> AMAQIDLNITCRFAGVFHVEKNGRYSISRTEAADLCKAFNSTLPTMAQMEKALSIGFETCRYGFIEGHVV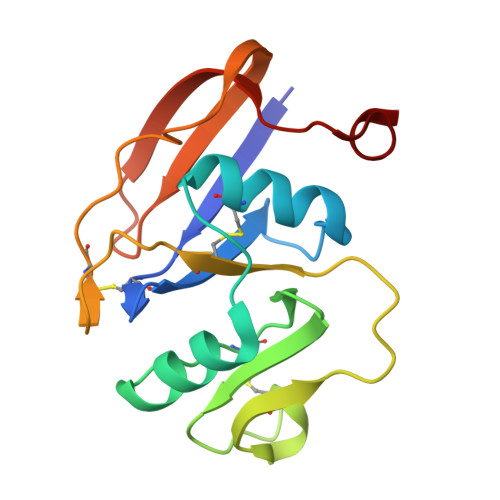IPRIHPNSICAANNTGVYILTSNTSQYDTYCFNASAPPEEDCTSVTDLPNAFDGPITITIVNRDGTRYVQKGEYRTNPEDIYP> DEHNKNMADIEAAFEGRVGVYAINTGSGKAYSYRANERFPLCSSFKAFLAAAVLKMDQDSPGVLLEKVNYHNRTME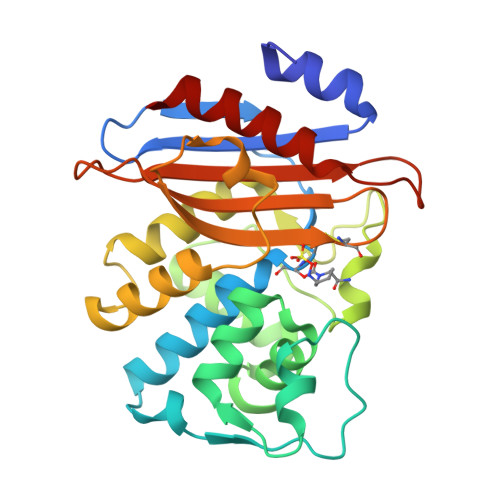PHSPITEKFQSQGMAVGELAAATLQYSDNGAANLLMEKYIKGPEGMTQFMNSIGDTKFRLDRWELDLNSAIPGDERDTSTPKAVAESLNKLISNTVLDNYHQEIFKKWMIGNTTGDNRIRAAVPDGWVVGDKTGTCGKYGTANDHAFILQGNNAAPLILSIYTTRKGEHMKHDDEVIAKAARIAIENVK>[2x]MK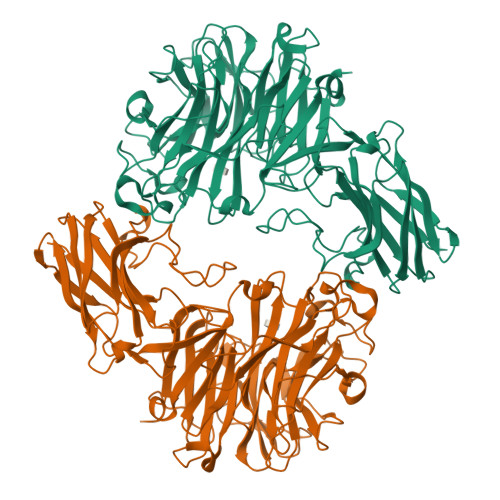KNLFLSIIFSFCVILQAFASDTVFVRETQIPVLIERQDNVLFMLRLNAKESHTLDEVVLNFGKDVNMSDIQSVKLYYSGTEARQNYGKNFFAPVSYISSHTPGKTLAANPSYSINKSQVNNPKRKVALKANQKLFPGINYFWISLQMKPDASLLDKVAAKIAAIKVDNKEALMHTVSPENIVHRVGVGVRHAGDDGSASFRIPGLVTTNKGTLLGVYDVRYNNSADLQEHVDIGLSRSVDGGKTWEKMRLPLAFGETGDLPAAQNGVGDPSILVDTKTNTVWVVAAWTHGMGNQRAWWSSYPGMDMNHTAQLVLSKSTDDGKTWSKPINITEQVKDPSWYFLLQGPGRGITMQDGTLVFPIQFIDSTRVPNAGIMYSKDRGETWKIHNYARTNTTEAQVAEVEPGVLMLNMRDNRGGSRAISTTKDLGKTWTEHSSSRKALQEPVCMASLISVKAKDNVLNKDILLFSNPNTVKGRHHITIKASLDGGVTWLPEHQVMLDEGEGWGYSCLTMIDKETIGILYESSVAHMTFQAVQLRDIIKHHHHHHHHHH> SGISLDNSYKMDYPEMGLCIIINNKNFHKSTGMTSRSGTDVDAANLRETFRNL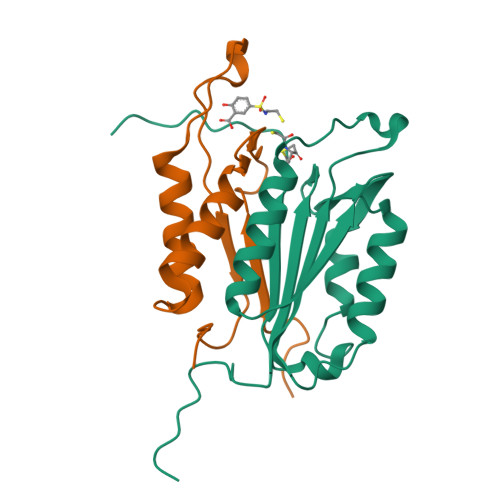KYEVRNKNDLTREEIVELMRDVSKEDHSKRSSFVCVLLSHGEEGIIFGTNGPVDLKKITNFFRGDRCRSLTGKPKLFIIQACRGTELDCGIET;> KIPVDADFLYAYSTAPGYYSWRNSKDGSWFIQSLCAMLKQYADKLEFMHILTRVNRKVATEFESFSFDATFHAKKQIPCIVSMLTKELYFYH>[2x]MSLDEDKTNDSAFHARLIAEVLEAYPDKARKRRQKHLNVAGQAEAEAQDAGEEGVMLSECDVKSNVKSVPGVMTIRGCAYAGSKGVVWGPVKDMVHISHGPVGCGQYSWSQRRNYYIGNTGVDSFVTMQFTSDFQEKDIVFGGDKKLEKIIDEIDELFPLAKGISVQSECPIGLIGDDIEAVSRKKKKEIGKTIVPVRCEGFRGVSQSLGHHIANDAIRD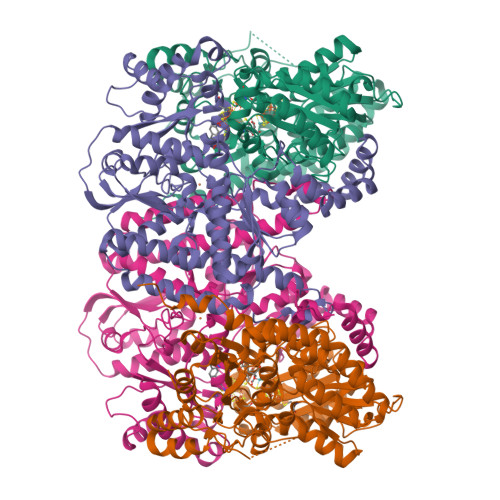WVFDGEDKHAAFETTPYDVNVIGDYNIGGDAWSSRILLEEMGLRVVGNWSGDATLAEIERAPKAKLNLIHCYRSMNYICRHMEEKYNIPWTEYNFFGPSQIAASLRKIAALFDEKIQEGAERVIAKYQPLVDAVIEKFRPRLAGKKVMLYVGGLRPRHVVNAYNDLGMEIVGTGYEFGHNDDYQRTGHYVREGTLIYDDVTGYELEKFIEGIRPDLVGSGIKEKYPVQKMGIPFRQMHSWDYSGPYHGYDGFAIFARDMDLAINNPVWSMFKAPWKNAA;>[2x]MPQNVDKILDHAPLFREPEYQEMLAGKAKLENMPPADKVVEIADWTKSWEYREKNFARESLSVNPAKACQPLGAVFVASGFERTMSFVHGSQGCVAYYRSHLSRHFKEPSSAVSSSMTEDAAVFGGLNNMVDGLANTYKLYDPKMIAVSTTCMAEVIGDDLHAFIQTAKGKGSVPEEFDVPFAHTPAFVGSHVTGYDNMLKGILEHFWKGRTPVPNRSVNIIPGFDGFAVGNNRELKRILGMMGVQYTILSDVSDQFDTPSDGEYRMYDGGTKIEAARDAVNADYTISLQEYCTPKTLEYCQSFGQKTASFHYPLGIGATDDLLQKLSEISGKPVPQELEMERGRLVDALADSQAYLHGKTYAIYGDPDFVYGMARFILETGGEPKHCLATNGSKAWEAQMQELFDSSPFGVGCKAWGGKDLWHMRSLLATEKVDLLIGNSYGKYLERDTDTPLIRLMFPIFDRHHHHRFPVWGYQGALRVLVTLLDKIFDKLDDDTIQAGVTDYSFDLTR> KRRQTS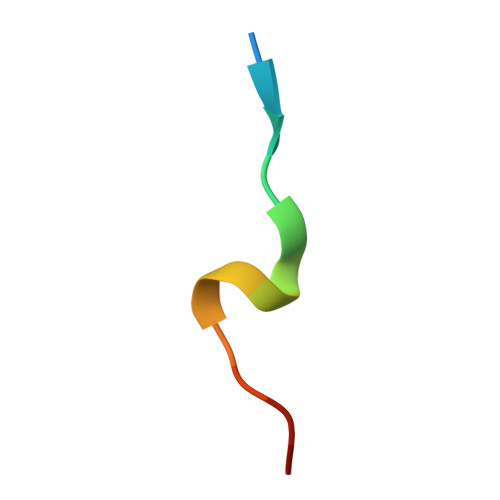MTDFYHSKR>MRSRRVDVMDVMNRLILAMDLMNRDDALRVTGEVREYIDTVKIGYPLVLSEGMDIIAEFRKRFGCRIIADFKVADIPETNEKICRATFKAGADAIIVHGFPGADSVRACLNVAEEMGREVFLLTEMSHPGAEMFIQGAADEIARMGVDLGVKNYVGPSTRPERLSRLREIIGQDSFLISPGAGAQGGDPGE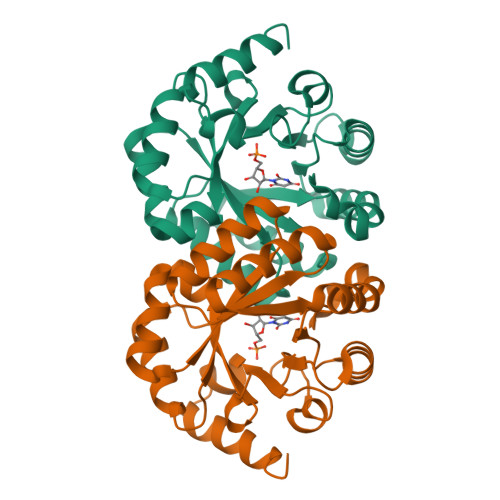TLRFADAIIVGRSIYLADNPAAAAAGIIESIKDLLNP[2x]> MRLLTWDVKDTLLRLRHPLGEAYATKARAHGLEVEPSALEQGFRQAYRAQSHSFPNYGLSHGLTSRQWWLDVVLQTFHLAGVQDAQAVAPIAEQLYKDFSHPCTWQVLDGAEDTLRECRTRGLRLAVISNFDRRLEGILGGLGLREHFDFVLTSEAAGWPKPDPRIFQEALRLAHMEPVVAAHVGDNYLCDYQGPRAVGMHSFLVVGPQALDPVVRDSVPKEHILPSLAHLLPALDCLEGSAENLYFQSHHHHHHDYK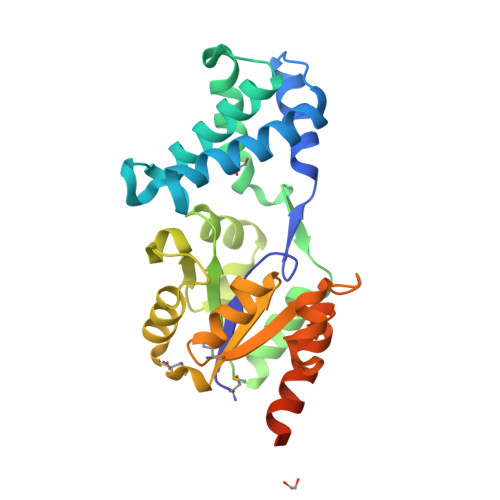DDDDK> MWKLLPAAGPAGGEPYRLLTGVEYVVGRKNCAILIENDQSISRNHAVLTANFSVTNLSQTDEIPVLTLKDNSKYGTFVNEEKMQNGFSRTLKSGDGITFGVFGSKFRIEYEPLVACSSCLDVSGKTALNQAILQLGGFTVNNWTEECTHLVMVSVKVTIKTICALICGRPIVKPEYFTEFLKAVESKKQPPQIESFYPPLDEPSIGSKNVDLSGRQERKQIFKGKTFIFLNAKQHKKLSSAVVFGGGEARLITEENEEEHNFFLAPGTCVVDTGITNSQTLIPDCQKKWIQSIMDMLQRQGLRPIPEAEIGLAVIFMTTKNYCDPQGHPSTGLKTTTPGPSLSQGVSVDEKLMPSAPVNTTTYVADTESEQADTWDLSERPKEIKVSKMEQKFRMLSQDAPTVKESCKTSSNNNSMVSNTLAKMRIPNYQLSPTKLPSINKSKDRASQQQQTNSIRNYFQPSTKKRERDEENQEMSSCKSARIETSCSLLEQTQPATPSLWKNKEQHLSENEPVDTNSDNNLFTDTDLKSIVKNSASKSHAAEKLRSNKKREMDDVAIEDEVLEQLFKDTKPELEIDVKVQKQEEDV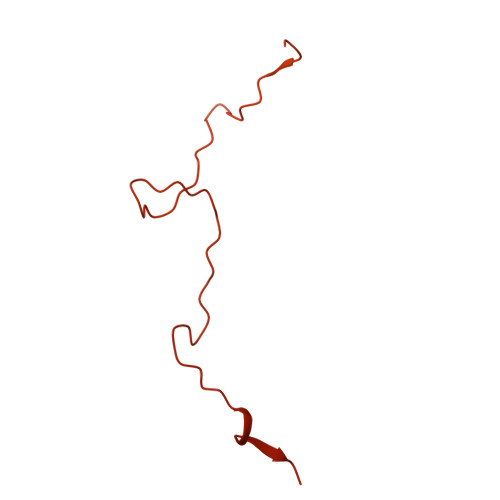NVRKRPRMDIETNDTFSDEAVPESSKISQENEIGKKRELKEDSLWSAKEISNNDKLQDDSEMLPKKLLLTEFRSLVIKNSTSRNPSGINDDYGQLKNFKKFKKVTYPGAGKLPHIIGGSDLIAHHARKNTELEEWLRQEMEVQNQHAKEESLADDLFRYNPYLKRRR>[2x]MHHHHHHMANRKLEKMASIDVHLRQLVPGKVSEDDKLVEYDALLLDRFLDILQDLHGEDLRETVQELYEHSAEYEGKHEPKKLEELGSVLTSLDPGDSIVIAKAFSHMLNLANLAEEVQIAYRRRIKKLKKGDFVDESSATTESDLEETFKKLVGDLNKSPEEIFDALKNQTVDLVLTAHPTQSVRRSLLQKHGRIRDCLAQLYAKDITPDDKQELDEALQR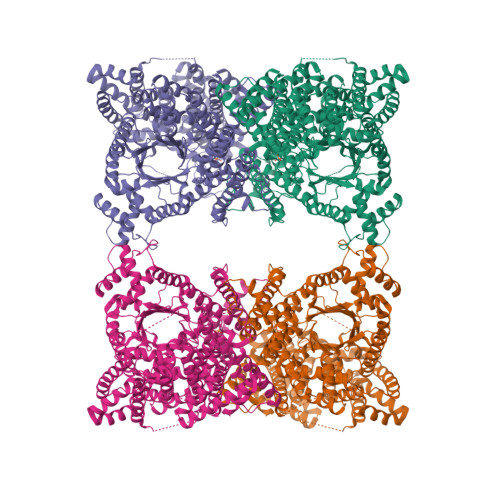EIQAAFRTDEIKRTPPTPQDEMRAGMSYFHETIWKGVPKFLRRVDTALKNIGIEERVPYNAPLIQFSSWMGGDRDGNPRVTPEVTRDVCLLARMMAATMYFNQIEDLMFEMSMWRCNDELRARADEVHANSRKDAAKHYIEFWKSIPTTEPYRVILGDVRDKLYHTRERAHQLLSNGHSDVPVEATFINLEQFLEPLELCYRSLCSCGDRPIADGSLLDFLRQVSTFGLSLVRLDIRQESDRHTDVLDAITTHLDIGSYREWSEERRQEWLLSELSGKRPLFGSDLPKTEEIADVLDTFHVIAELPADSFGAYIISMATAPSDVLAVELLQRECRVKQPLRVVPLFEKLADLEAAPAAVARLFSVDWYKNRINGKQEVMIGYSDSGKDAGRLSAAWQLYKAQEELVKVAKEYGVKLTMFHGRGGTVGRGGGPTHLAILSQPPDTINGSLRVTVQGEVIEQSFSEEHLCFRTLQRFTAATLEHGMRPPISPKPEWRALLDEMAVVATEEYRSVVFQEPRFVEYFRLATPELEYGRMNIGSRPSKRKPSGGIESLRAIPWIFAWTQTRFHLPVWLGFGSAIRHVIEKDVRNLHMLQDMYQHWPFFRVTIDLIEMVFAKGDPGIAALYDKLLVSEELWPFGEKLRANFEETKKLILQTAGHKDLLEGDPYLKQRLRLRDSYITTLNVCQAYTLKRIRDPSYHVTLRPHISKEIAESSKPAKELIELNPTSEYAPGLEDTLILTMKGIAAGLQNTG> AQTVPYGIPLIKADKVQAQGFKGANVKVAVLDTGIQASHPDLNVVGGASFVAGEAYNTDGNGHGTHV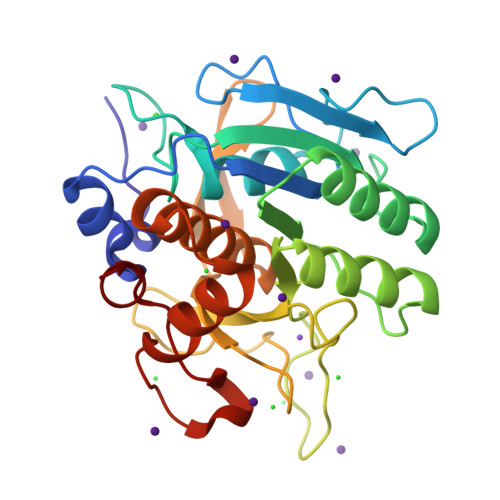AGTVAALDNTTGVLGVAPSVSLYAVKVLNSSGSGSYSGIVSGIEWATTNGMDVINMSLGGASGSTAMKQAVDNAYARGVVVVAAAGNSGNSGSTNTIGYPAKYDSVIAVGAVDSNSNRASFSSVGAELEVMAPGAGVYSTYPTNTYATLNGTSMASPHVAGAAALILSKHPNLSASQVRNRLSSTATYLGSSFYYGKGLINVEAAAQ>MAILDSAGVTTVTENGGGEFVDLDRLRRRKSRSDSSNGLLLSGSDNNSPSDDVGAPADVRDRIDSVVNDDAQGTANLAGDNNGGGDNNGGGRGGGEGRGNADATFTYRPSVPAHRR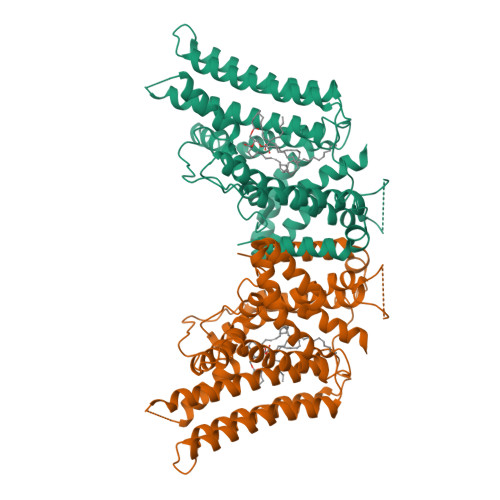ARESPLSSDAIFKQSHAGLFNLCVVVLIAVNSRLIIENLMKYGWLIRTDFWFSSRSLRDWPLFMCCISLSIFPLAAFTVEKLVLQKYISEPVVIFLHIIITMTEVLYPVYVTLRCDSAFLSGVTLMLLTAIVWLKLVSYAHTSYDIRSLANAADKANPEVSYYVSLKSLAYFMVAPTLCYQPSYPRSACIRKGWVARQFAKLVIFTGFMGFIIEQYINPIVRNSKHPLKGDLLYAIERVLKLSVPNLYVWLCMFYCFFHLWLNILAELLCFGDREFYKDWWNAKSVGDYWRMWNMPVHKWMVRHIYFPCLRSKIPKTLAIIIAFLVSAVFHELCIAVPCRLFKLWAFLGIMFQVPLVFITNYLQERFGSTVGNMIFWFIFCIFGQPMCVLLYYHDLMNRKGSMSGPHHHHHH[2x]>[2x]GPKLLQILNVRVVGSGERVVVLSHGFGTDQSAWSRVLPYLTRDHRVVLYDLVCAGSVNPDHFDFRRYDNLDAYVDDLLAILDALRIPRCAFVGHSVSAMIGILASIRRPDLFAKLVLIGASPRFLNDSDYHGGFELEEIQQVFDAMGANYSAWATGYAPLAVGADVPAAVQEFSRTLFNMRPDISLHVCQTVFKTD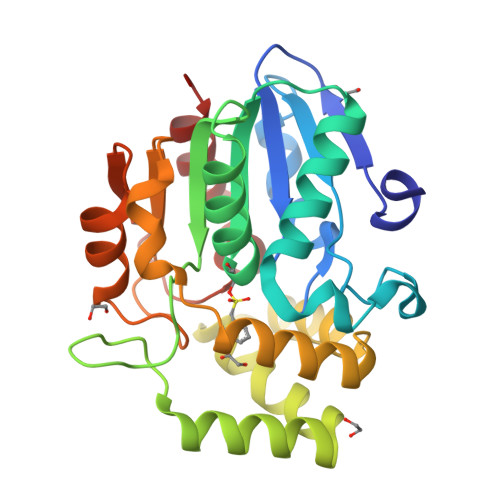LRGVLGMVRAPCVVVQTTRDVSVPASVAAYLKAHLGGRTTVEFLQTEGHLPHLSAPSLLAQVLRRALARY> MSWQTYVDDHLMCDVAGNRLTAAAILGQDGSVWAQSNNFPQVKPEEIQGIKDDFTTPGTLAPTGLFLGGNKYMVIQGEPNAVIRGKKG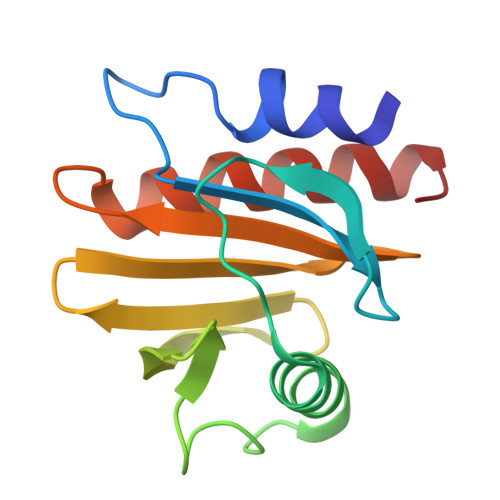AGGVTIKKTTLALVFGIYDEPMTPGQCNMVVENLGEYLIESGL>[4x]SIYKVENRHDYGTKGTKVDILTGSGRVPSRILDAPVVQFKESTFEYKDKSYGTKHEESKGNWNMKGHQFISTPAKQVNLRAIFINNANTAPPASMESELDISMDKFASDVKQLGVDFNVSGKPILINQFGPPIKKFQGGGRGGRGGRGSRGGRGGRGAPSGPPTFETSPGEISLLNLLENIPSNTYILYVLRRGNDSAVYDRLKYITDLKFGALNSCVVWDNFKKNSIQYNSNVVMKMNLKLLGSNHSLSIENNKLLIDKESNLPILVLGSDVTHYPEKDQNSIASLVGSYDDKFTQFPGDYMLQDGPGEEIITNVGSLMLNRLKIYQKHNNGKLPTKIMYFRDGVSVDQFSQ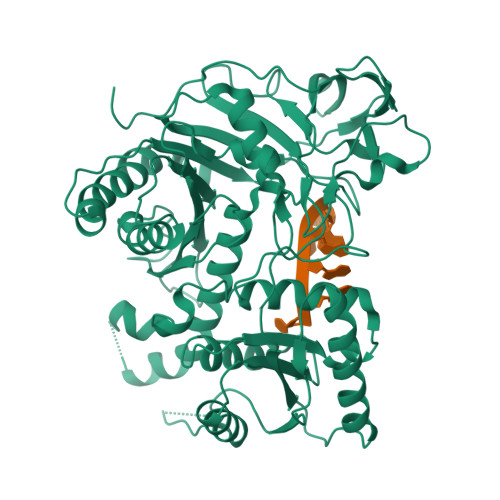VVKIEVKSIKESVRKFGPQLNGGNKYDPPVTCIATVKRNQVRFIPIQENAKNEKGEEVAVQSMGNVMPGTVVDRGITSVAHFDFFIQSHQALKGTGVPCHYWCLYDENQSTSDYLQEICNNLCYIFGRSTTSVKVPAPVYYADLLCTRATCFFKAGFELNMAQAPKEKGSKDQPTVSKNVLLPQVNDNIKSVMYYI> EMPVDRILEAELAVEQKSDQGVEGPGGTGGSGSSPNDPVTNICQAADKQLFTLVEWAKRIPHFSSLPLDDQVILLRAGWNELLIASFSHRSIDVRDGILLATGLHVHRNSAHSAGVGAIFDRVLTELVSKMRDMRMDKTELGCLRAIILFNPDAKGLSNPSEVEVLREKVYASL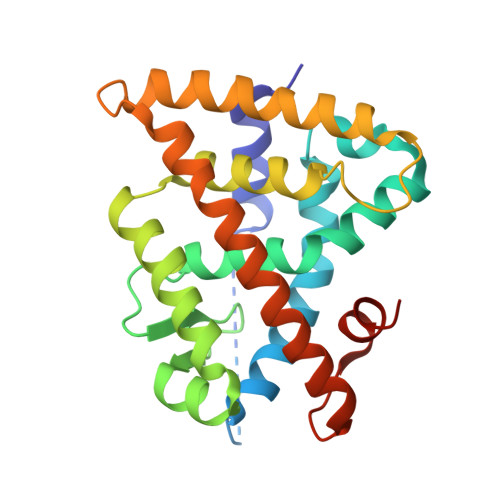ETYCKQKYPEQQGRFAKLLLRLPALRSIGLKCLEHLFFFKLIGDTPIDTFLMEMLEAPHQLA>AETVESCLAKPHTENSFTNVWKDDKTLDRYANYEGCLWNATGVVVCTGDETQCYGTWVPIGL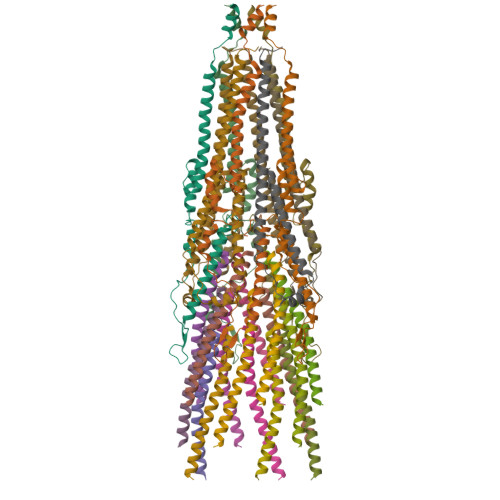AIPENEGGGSEGGGSEGGGSEGGGTKPPEYGDTPIPGYTYINPLDGTYPPGTEQNPANPNPSLEESQPLNTFMFQNNRFRNRQGALTVYTGTVTQGTDPVKTYYQYTPVSSKAMYDAYWNGKFRDCAFHSGFNEDPFVCEYQGQSSDLPQPPVNAGGGSGGGSGGGSEGGGSEGGGSEGGGSEGGGSGGGSGSGDFDYEKMANANKGAMTENADENALQSDAKGKLDSVATDYGAAIDGFIGDVSGLANGNGATGDFAGSNSQMAQVGDGDNSPLMNNFRQYLPSLPQSVECRPFVFGAGKPYEFSIDCDKINLFRGVFAFLLYVATFMYVFSTFANILRNKES[5x];>[15x]MKKSLVLKASVAVATLVPMLSFAAEGDDPAKAAFNSLQASATEYIGYAWAMVVVIVGATIGIKLFKKFTSKAS;>MPVLLGIPLLLRFLGFLLVTLFGYLLTFLKKGFGKIAIAISLFLALIIGLNSILVGYLSDISAQLPSDFVQGVQLILPSNALPCFYVILSVKAAIFIFDVKQKIVSYLDWDK[5x]>[2x]MAGNETIETFLDGLASSAPTPGGGGAAAISGAMGAALVSMVCNLTIGKKKYVEVEADLKQVLEKSEGLR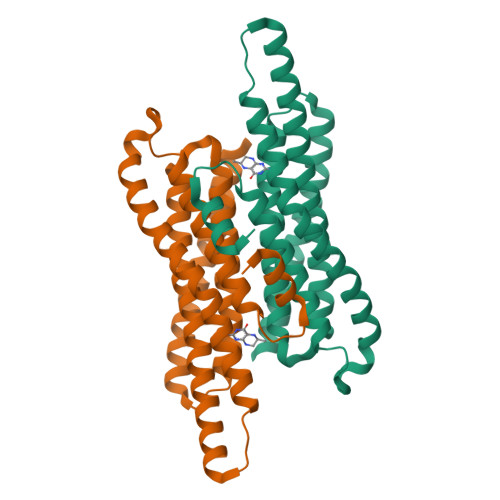RTLTGMIADDVEAFDAVMGAYGLPKNTDEEKAARAAKIQEALKTATDVPLACCRVCREVIDLAEIVAEKGNLNVISDAGVAVLSAYAGLRSAALNVYVNAKGLDDRAFAEERLKELEGLLAEAGALNERIYETVKSKVNLEHHHHHH Here, we discovered a three-component monooxygenase system consisting of AibH1H2, AibG, and AibF for Aib hydroxylation in a Rhodococcus wratislaviensis strain possessing an oxygen-dependent Aib catabolic pathway not dependent on α,α-dialkylglycine decarboxylase. AibH1H2, a non-heme diiron enzyme, acts as the terminal oxygenase in the three-component monooxygenase system to produce α-methyl-d-serine (D-MeSer). All previously reported amino acid hydroxylases that form hydroxy groups on an aliphatic C–H bond belong to the Fe(II)/α-ketoglutarate-dependent dioxygenase (2OGDO) superfamily, but AibH1H2 belongs to the amidohydrolase superfamily (AHS). Thus, AibH1 and H2 are α′ and α subunits forming an α2α′2 heterotetrameric complex that act as the hydroxylase component in the Aib monooxygenase.

AibH1H2 has a heterotetrameric structure of AibH1 and AibH2 subunits, and each subunit has the characteristic (β/α)8-barrel (TIM-barrel) fold present in all members of the AHS. Clear electron density is observed in the crystal structures of AibH1 and AibH2, which is consistent with metal ion occupancy. A metal content analysis indicated the presence of 1.96 Fe and 0.76 Zn per AibH1H2. Moreover, the positions of the metal-coordinating amino acid residues in AibH2 are very similar to that in PtmU3—a non-heme diiron hydroxylase belonging to AHS30—thereby indicating that AibH2 also has a diiron catalytic center. In AibH2, the two Fe ions are coordinated by side-chains of three histidine and three carboxylate residues (Asp25H2, His27H2, His211H2, Glu265H2, Asp337H2, and His340H2), an ethylene glycol, and an oxygen atom. AibH1 contains one Zn ion coordinated by side-chains of two histidine and three carboxylate residues (Asp24H1, His26H1, His201H1, Glu255H1, and Asp328H1). Thus, the AibH1H2 heterotetrameric complex contains two catalytic AibH2 subunits, each with a diiron center, and two AibH1 subunits, each containing a zinc ion. Although the His331 residue in AibH1 corresponding to His340 in AibH2 is conserved, the Asp residue corresponding to Asp342 in AibH2 is missing in the mononuclear AibH1. The acidic residue (Asp or Glu) at this position is conserved only in AHS enzymes with binuclear centers. So, the acidic residue is important for binding an additional metal ion to form a binuclear catalytic center in AHS enzymes.

> DGVPAVVDCDVHAVLPSPHSLIPYLDEYWADQLVAQLAPTYEPNYHPRGSAIAQHSDASVDENGRAATTAENLVKDVFADGFTDFAVVNCLYGVQQIHQPRREMAHARALNHWIANEWLDKDDRLRASIVVPQGSPRAAAEEIDFWSGDKRFVQVLLLGQSELLYGREINWPIWEAAEAAGLPVTLHIGGVFRQAPTSVGWPASHLEWYVGQQSNIEAQLNSIISEGILQKFPKTKILLSELGFNWLPPFMWKFDKLWKSYRPDIPWVQESPLELIREHVRVTTSPSDGAEEAGRLDSIVDRLGSDRMLVYSSDYPHKHHSGPRDIENGTHSPELLDRIYRRNAFDLYNLVVPS;> MTIIEHGSLGTLPAPSVTTGIVDADIHPVPQDGALEPYLDDRWKKHIREYGVRTTTGLQFISEYPQMYGGAMRADAWPESGYPGSDRELLRTQLLDKHNIQLGVLQCLAPGGQTLNPAGQALNQELAAALCRATNDWQLEHLVYPDPRMRAAIPVTFETPDYAVAEIERVGADPGVVAVLGTSKTLEPLGSRKYWPIYEASVAQNLPIQFHLSQGGGHANTGTGWTSYHTEYHTGHVQSFQSQLLSLVLSGTFDRFPTLKVMFVEGNVAHFAPLIQRMDYTWETLRGELPDLQRKPSEYIRDHIWASTQPIDEPEKPEHLAELLEEFCGDNVVFATDYPHFDFDDPETAFPRSFPVDLRDKILRGNGMRFFGVTNQAD>RWGS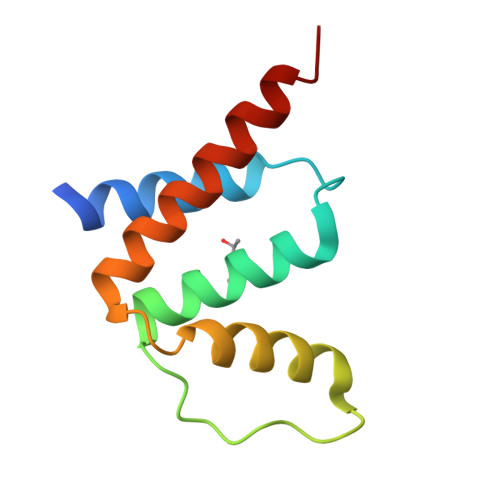MGLQEEFEEFAEKAKTLPDTISNEDKLLLYGLYKQATVGPVTTGRPGIFNLKDRYKWDAWKAVEGKSKEEAMADYITKVKQLLEEASASTS[4x]ethyl (2Z)-2-hydroxyimino-3-oxidanylidene-butanoate 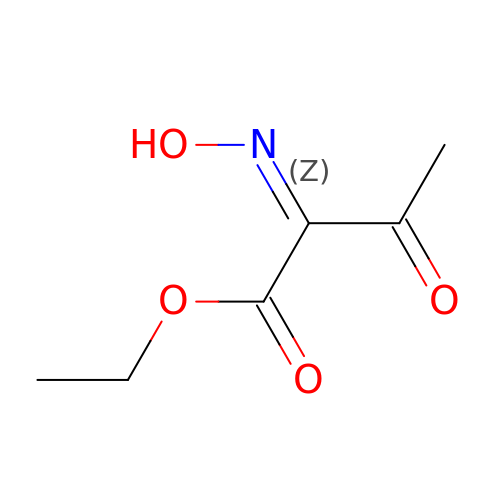| C6 H9 N O4 | IACSYDRIOYGJNH-ALCCZGGFSA-N> SITENTSWNKEFSAEAVNGVFVLCKSSSKSCATNDLARASKEYLPASTFKIPNAIIGLETGVIKNEHQVFKWDGKPRAMKQWERDLTLRGAIQVSAVPVFQQIAREVGEVRMQKYLKKFSYGNQNISGGI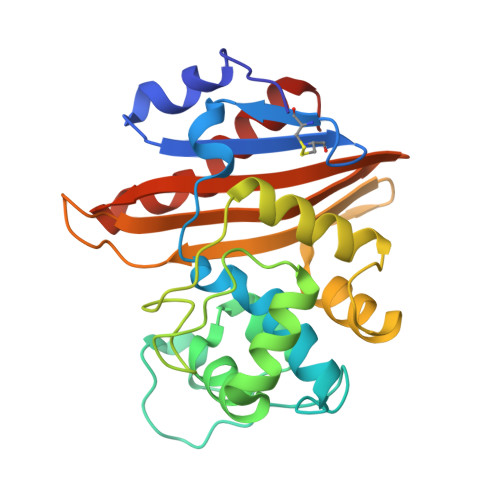DKFWLEGQLRISAVNQVEFLESLYLNKLSASKENQLIVKEALVTEAAPEYLVHSKTGFSGVGTESNPGVAWWVGWVEKETEVYFFAFNMDIDNESKLPLRKSIPTKIMESEGIIGG>[4x]GGCUAGCUGGAGGGGCGCCAGUUCGCUGGUGGUUGGGUGCGGUCGGCUAGCC

The Chili RNA aptamer mimics large Stokes shift fluorescent proteins and exhibits high affinity for 3,5-dimethoxy-4-hydroxybenzylidene imidazolone (DMHBI) derivatives to elicit green or red fluorescence emission. The Chili RNA folds into a single coaxial helical stack with a length of ~70 Å that contains two A-form duplexes P1 and P2 that are separated by the central fluorophore binding domain (FBD). The P1 stem transitions via a base triple into a two-tiered G-quadruplex, which constitutes the core of the FBD. The ligand is immobilized by π-stacking between an unusual G14:G31 base pair and the T2 quartet.

The 52-nt Chili RNA aptamer was co-crystallized with two of its cognate ligands, DMHBO+ and DMHBI+. Crystals were derivatized with iridium(III) hexammine (by soaking or co-crystallization), experimental phases were obtained by single-wavelength anomalous dispersion (SAD), and the initial models were used for molecular replacement (MR) with native datasets.> SNAMSKADIIVGIQWGDEGKGKVVDKLCENYDFVCRSAGGHNAGHTIWVNGVRYALHLMPSGVLHPRCINIIGNGVVVSPEVLIAEMAQFENLKGRLYISDRAHLNLKHHSLIDIAKEKLKGKNAIGTTGKGIGPSYADKINRTGHRVGELLEPQRLCEALIKDFEANKTFFEMLEIEIPSAEELLADLKRFNEILTPYITDTTRMLWKALDEDKRVLLEGAQGSMLDIDHGTYPYVTSSSTISAGTLTGLGLNPKEAGNIIGIVKAYATRVGNGAFPTEDKGEDGEKIAQIG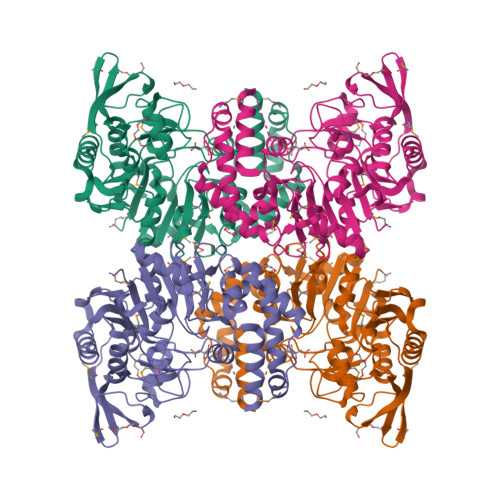KEIGVSTGRKRRCGWFDAVAVRYTARLNGLDALSLMKLDVLDGFEKIKICRAYEYKGMEIDYIPSDLENVQPIYEEMDGWDKVFGIKDYDLLPENAKKYIARLEELAGVKVKYISTSPERDDTIIL3-[(1-methyl-1H-pyrrolo[2,3-b]pyridin-3-yl)amino]pyridine-4-carboxylic acid | 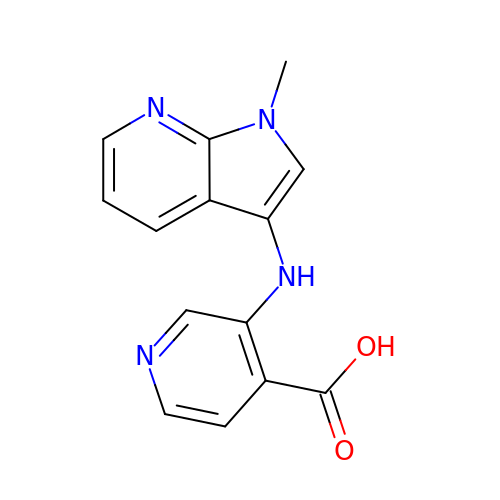C14 H12 N4 O2 | RBGNHCYGFBRIRO-UHFFFAOYSA-N>DPWQECMDYAVTLARQAGEVVCEAIKNEMNVMLKSSPVDLVTATDQKVEKMLISSIKEKYPSHSFIGEESVAAGEKSILTDNPTWIIDPIDGTTNFVHRFPFVAVSIGFAVNKKIEFGVVYSCVEGKMYTARKGK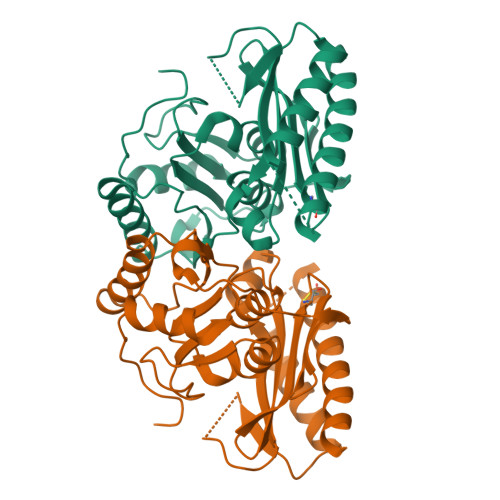GAFCNGQKLQVSQQEDITKSLLVTELGSSRTPETVRMVLSNMEKLFCIPVHGIRSVGTAAVNMCLVATGGADAYYEMGIHCWDVAGAGIIVTEAGGVLMDVTGGPFDLMSRRVIAANNRILAERIAKEIQVIPLQRDDE[2x]> MLKRFPTPILKVYWPFFVAGAAVYYGMSKAA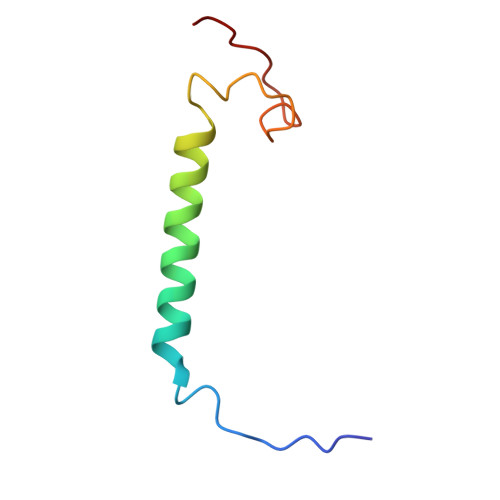DLSSNTKEFINDPRNPRFAKGGKFVEVD> KAQQEERLDEINKQFLDDPKYSSD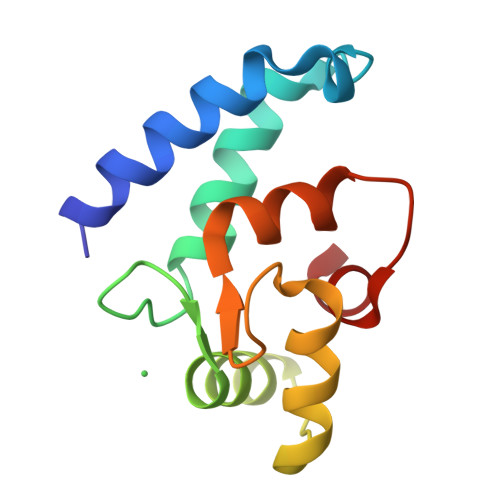EDLPSKLEGFKEKYMEFDLNGNGDIDIMSLKRMLEKLGVPKTHLELKKLIGEVSSGSGETFSYPDFLRMMLGKRSAILKMILM> A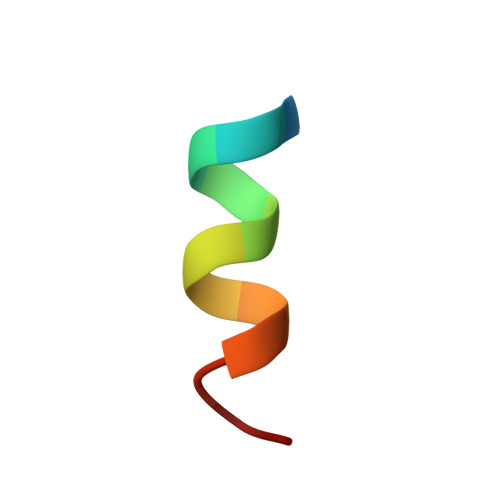TRELDELMASLS> MAAASFGQTKIPRGNGPYSVGCTDLMFDHTNKGTFLRLYYPSQDNDRLDTLWIPNKEYFWGLSKFLGTHWLMGNILRLLFGSMTTPANWNSPLRPGEKYPLVVFSHGLGAFRTLYSAIGIDLASHGFIVAAVEHR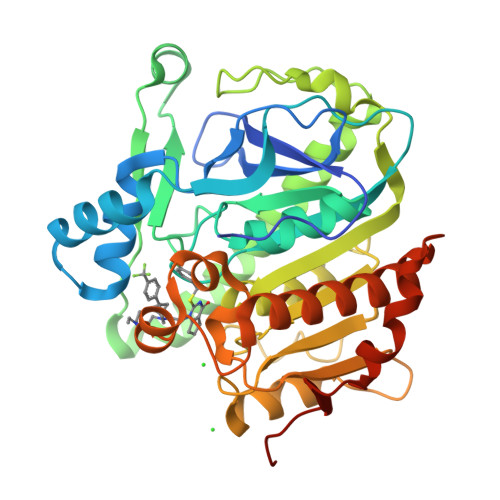DRSASATYYFKDQSAAEIGDKSWLYLRTLKQEEETHIRNEQVRQRAKECSQALSLILDIDHGKPVKNALDLKFDMEQLKDSIDREKIAVIGHSFGGATVIQTLSEDQRFRCGIALDAWMFPLGDEVYSRIPQPLFFINSEYFQYPANIIKMKKCYSPDKERKMITIRGSVHQNFADFTFATGKIIGHMLKLKGDIDSNVAIDLSNKASLAFLQKHLGLHKDFDQWDCLIEGDDENLIPGTNINTTNQHHHHHH~{N}-(4,4-dimethyl-2-prop-1-ynyl-3,1-benzoxazin-6-yl)-2-[3-methoxy-5-(7-methoxyquinolin-4-yl)oxy-pyridin-2-yl]ethanamide | C31 H28 N4 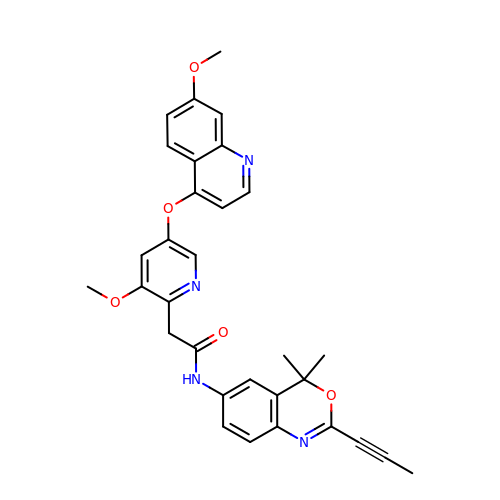O5 | RBASQIFWXZMGHR-UHFFFAOYSA-N>[2x]MSLTNGEENEEVLFCEKAKLLIFDSDTKGYTSRGVGELKLLRKKDDKGKVRVLCRSEGMGHVLLNTSVVKSFKYQPIDADNENLIKWPIITDGKLETFIIKVKQKAD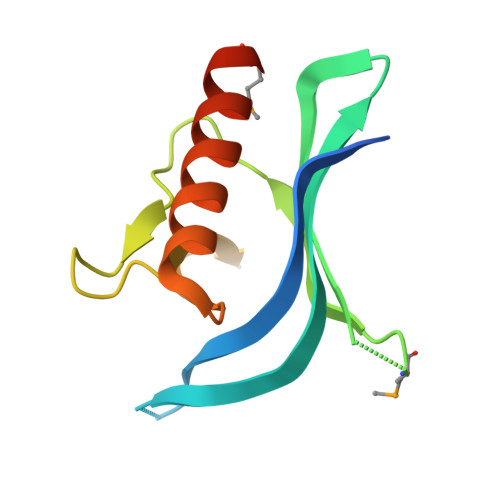GRRLVGAVADAQQAMEGHHHHHH2-(11-oxo-10,11-dihydro-5H-dibenzo[b,e][1,4]diazepin-3-yl)benzamide | C20 H15 N3 O2 | 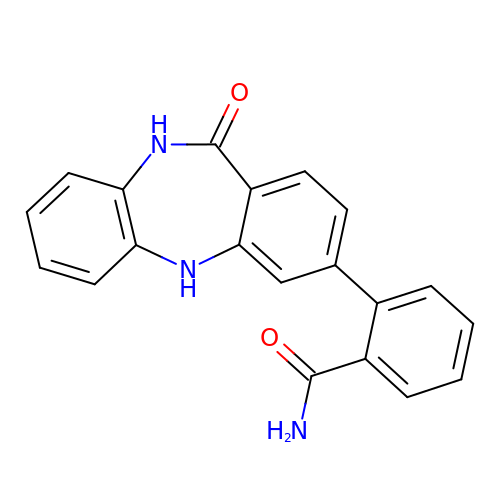XLSKYJYTEGNOBA-UHFFFAOYSA-N> MTILTDENYVDIAEKAILK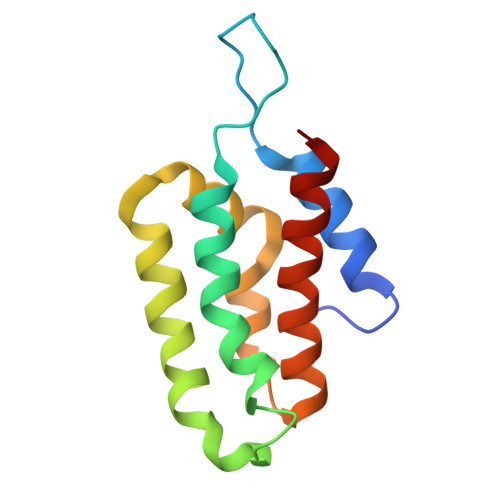LERNTRNRKNPDAFFLTTSKLRNLLSLTSTLFDESKVKEYDALLDRIAYLRVQFVYQAGREIAVKDLIEKAQILEALKEIKDRETLQRFCRYMEALVAYFKFYGGKD>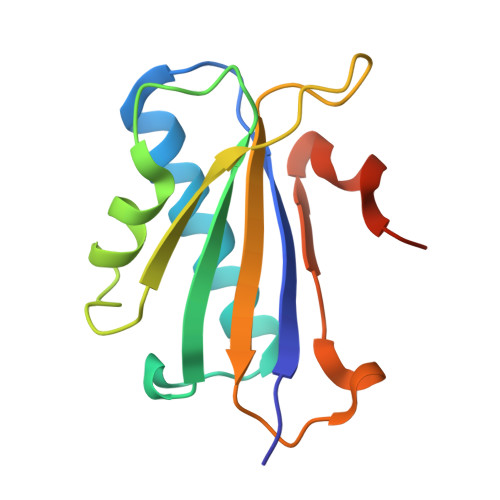 GSVRGIRGAITVEEDTPAAILAATIELLLKMLEANGIQSYEELAAVIFTVTEDLTSAFPAEAARLIGMHRVPLLSAREVPVPGSLPRVIRVLALWNTDTPQDRVRHVYLNEAVRLRPDLESAQLE> ASRSQAEDVRVEGSFPVTMLPGDGVGPELMHAVKEVFKAAAVPVEFQEHHLSEVQNMASEEKLEQVLSSMKENKVAIIGKIHTPMEYKGELASYDMRLRRKLDLFANVVHVKSLPGYMTRHNNLDLVIIREQTEGEYSSLEHESARGVIECLKIVTRAKSQRIAKFAFDYATKKGRGKVTAVHKANIMKLGDGLFLQCCEEVAELYPKIKFETMIIDNCCMQLVQNPYQFDVLVMPNLYGNIIDNLAAGLVGGAGVVPGESYSAEYAVFETGARHPFAQAVGRNIANPTAMLLSASNMLRHLNLEYHSSMIADAVKKVIKVGKVRTSDMGGYATCHDFTEEICRRVKD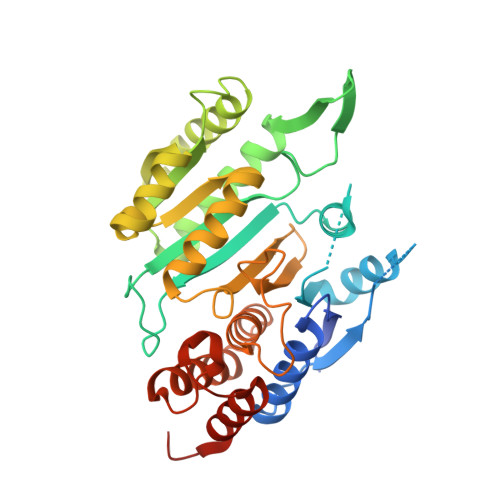LDENLYFQ>[2x]GSHMASTYLSDMDWSSATHGDIDKTKTVQKDAPFTTGNKGEHTKISLLTSDDKVKYFDKGIGTVADSPSVISYDISGQGFEKFETYIGIDQSANSSRSDHAVVDRIEIEIDGKVVYSSSVTNPEGF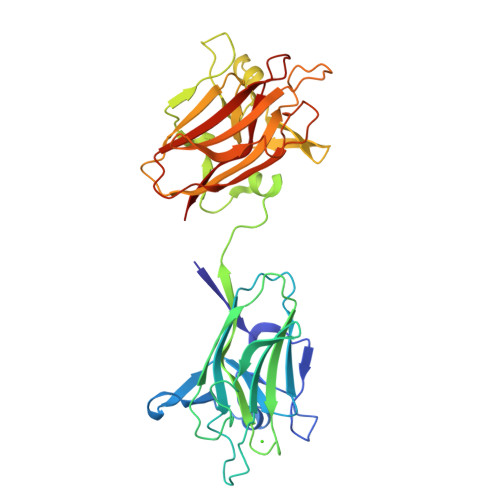RYNTQAQFISVTIPQNAKKISLKSFAGEHTWGDEVVFADAKLIKTVSTQTITPDLLNKGINGGVYLSDLEWVDATHGDDDKSKTVQKDKPFTPGNNGSNNKIKLLIDGKEVEFNKGLGTVASNPSSIKYDVSGANVTRFISYVGIDRSANHLNSDYADIQKFEVVADGKVIYSSDSKYPKGIKYDTSAFLVDVEIPKDTQTIELKSYSGKHTWADELVLGGALFMANG>GHMNSKNTICLWYDSAALEAATFYAETFPDSAVLAVHRAPGDYPSGKEGDVLTVEFRVMGIPCLGLNGGPAFRHSEAFSFQVATDDQAETDRLWNAIVDNGGEESACGWCRDKWGISWQITPRVLSEAIASPDR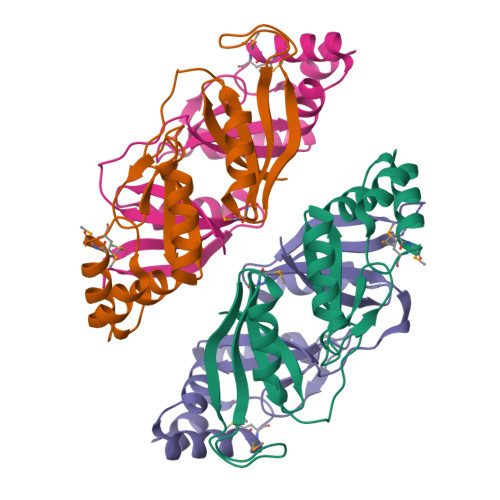AAARRAFEAMMTMGRIDIATIEKAFKGGS[4x]> VYFLKKKKNKILTIALVASLAASVSFGSVLYYSFSDNHISFDT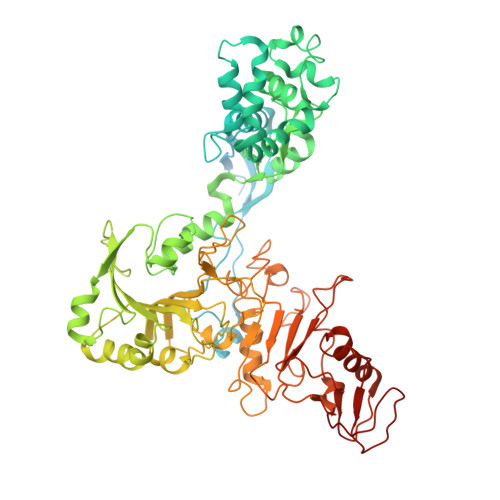SSNGITDAELAPINNAINDAIVSNRDNKLKPSEEKIIKETEKKIEEKIIIPPAKKEEKIEAAKPIPKPVVRKPETKITSPKITRRKQTITIAGIEVEAEIEGPPGFVTHQRDKDRKISNPTKPYQNHTVNKILSVKVTDKLKEQVAKDALSGGNGYDEGVGLFNNSIFNVFKEEFNSGKELNDILSSLESVARQNSGAFQNTLERYKKMLDSNNVINFLKSEAQKEYPKLKSKFQTKNQEYIWLIANLDQSKFTKIASTSEKYLEKGLTISPRSAFINEAGEIDSNGWGPPDEYNTVTSRLRRDNSEYRVFDYDEYYSRSSDRIANGTYPGWVKEDVSEPYSKKYNFKASDGIRFSKLERINPNPAKGKLNSGLVLDLDVSNDEAYRRSKELIEKLQKDGEQITSYRIKNMGEKNSDQAFKDILGALPKDIQQLELFFSDKATNTASLIALENKNIKELSLYTSGNSLKKAWSYNPLALRNTTWINTIDYNVSAEYSSHDKITTRITFNTLAFDQEDFSNGSYERINDGLRMVYYARNNEPFFQGGHGPGLEPDKKLGQNSYPTGLDFSRVTGIKSLKGLRFDDDLDTSNEPRKITELTLYNNESYFEISSDELNEANLQHLSTGEGNPEKPKIHFSNGNNTTSIRISGKTLLSDEGRRNLDKYFEYNESLRNSGKQIQIPNGSDELKKQLEGWGYKVSTASDRSFT>MNHKVHHHHHHIEGRHMELSPDGNLKTTITIGDRLTYDITCNGRQILTPSPISMTLDNGTVWGENA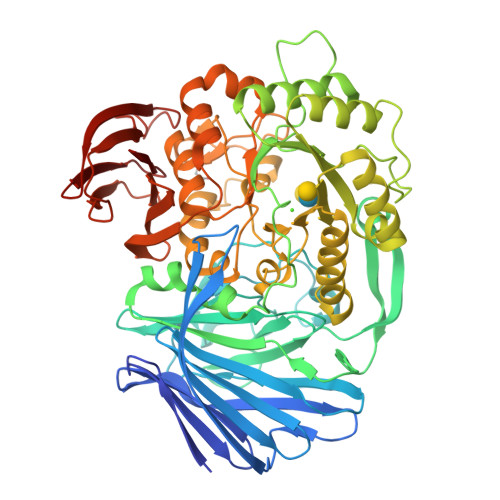KLSGTSRKSVDEMIPSPFYRASELRNHYNGLTLRFKKDWNVEFRAYNDGIAYRFVNQGKKPFRVVTEVSDYCFPSDMTASVPYVKSGKDGDYNSQFFNSFENTYTTDKLSKLNKQRLMFLPLVVDAGDGVKVCITESDLENYPGLYLSASEGANRLSSMHAPYPKRTVQGGHNQLQMLVKEHEDYIAKVDKPRNFPWRIAVVTTTDKDLAATNLSYLLGAPSRMSDLSWIKPGKVAWDWWNDWNLDGVDFVTGVNNPTYKAYIDFASANGIEYVILDEGWAVNLQADLMQVVKEIDLKELVDYAASKNVGIILWAGYHAFERDMENVCRHYAEMGVKGFKVGFMDRDDQEMTAFNYRAAEMCAKYKLILDLHGTHKPAGLNRTYPNVLNFEGVNGLEQMKWSSPSVDQVKYDVMIPFIRQVSGPMDYTQGAMRNASKGNYYPCYSEPMSQGTRCRQLALYVVFESPFNMLCDTPSNYMREPESTAFIAEIPTVWDESIVLDGKMGEYIVTARRKGDVWYVGGITDWSARDIEVDCSFLGDKSYHATLFKDGVNAHRAGRDYKCESFPIKKDGKLKVHLAPGGGFALKIK[2x]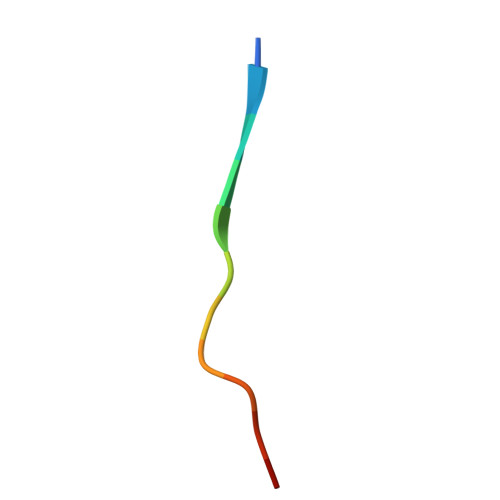> SWYSYPPPQRAV> MDEAVQFSNASYEAVIMENLALGTEIVRVQAYSIDNLNQITYRFDAYTSAQAKALFKIDAITGVITVKGLVDREKGDFYTLTVVADDGGPKVDSTVKVYITVLDENDNSPRFDFTSDSAISVPEDCPVGQRVATVKARDPDAGSNGQVVFSLASGNIAGAFEIITSNDSIGEVFVAKPLDREELDHYILKVVASDRGTPPRKKDHILQVTILDVNDNPPVIESPFGYNVSVNENVGGGTSVVQVRATDRDIGINSVLSYYITEGNEDMT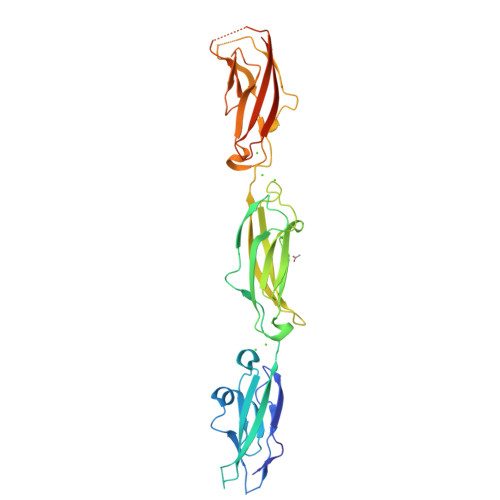FRMDRISGEIATRPAPPDRERQNFYHLVVTVEDEGTPTLSATTHVYVTIVDENLEHHHHHH ERDRP-0519 is a potent nonnucleoside inhibitor active against measles virus (MeV) and other Morbilliviruses. Conversely, polymerase inhibitors like ERDRP-0519 show greater promise due to the high conservation of the L-P complex across MeV strains. Here we report cryo-EM structures of the compound bound to MeV polymerase complexes at 2.73 Å and 2.48 Å resolution, revealing a unique binding pocket in the RdRp palm subdomain that overlaps the catalytic GDN motif. Structural analysis revealed that ERDRP-0519 binds to the palm subdomain of the RdRp, targeting the catalytic GDN motif and a nearby hydrophobic channel.

To test this, we assembled the MeV ternary polymerase complex14 with ERDRP-0519 and analyzed it by cryo-EM. The maps revealed two complexes: Lcore-P and Lfull-P-C, with clear ERDRP-0519 density on the L protein. Contrary to predictions, ERDRP-0519 was observed binding within the RdRp domain rather than at the predicted PRNTase site. First, it inhibits the catalytic center by interacting with residue D773 in the GDN motif. The piperidine group displaces D773, creating space for hydrophobic interaction that directly impairs active site function. A strong hydrogen bond (2.8 Å) forms between the compound’s carboxyl group in the linker and residue W671 of the L protein. ERDRP-0519 failed to inhibit the W671F mutant, confirming W671’s essential role in binding and antiviral activity. The central ring forms strong hydrophobic interactions with residue Y667, so any changes at this position are likely to cause steric clashes, disrupting binding. Additionally, the trifluoromethylated pyrazole group fits precisely into a hydrophobic pocket, engaging six surrounding residues and forming more interactions than any other part of the molecule.

> MDSLSVNQILYPEVHLDSPIVTNKIVAILEYARVPHAYSLEDPTLCQNIKHRLKNGFSNQMIINNVEVGNVIKSKLRSYPAHSHIPYPNCNQDLFNIEDKESTRKIRELLKKGNSLYSKVSDKVFQCLRDTNSRLGLGSELREDIKEKVINLGVYMHSSQWFEPFLFWFTVKTEMRSVIKSQTHTCHRRRHTPVFFTGSSVELLISRDLVAIISKESQHVYYLTFELVLMYCDVIEGRLMTETAMTIDARYTELLGRVRYMWKLIDGFFPALGNPTYQIVAMLEPLSLAYLQLRDITVELRGAFLNHCFTEIHDVLDQNGFSDEGTYHELIEALDYIFITDDIHLTGEIFSFFRSFGHPRLEAVTAAENVRKYMNQPKVIVYETLMKGHAIFCGIIINGYRDRHGGSWPPLTLPLHAADTIRNAQASGDGLTHEQCVDNWKSFAGVKFGCFMPLSLDSDLTMYLKDKALAALQREWDSVYPKEFLRYDPPKGTGSRRLVDVFLNDSSFDPYDVIMYVVSGAYLHDPEFNLSYSLKEKEIKETGRLFAKMTYKMRACQVIAENLISNGIGKYFKDNGMAKDEHDLTKALHTLAVSGVPKDLKESHRGGPVLKTYSRSPVHTSTRNVRAAKGFIGFPQVIRQDQDTDHPENMEAYETVSAFITTDLKKYCLNWRYETISLFAQRLNEIYGLPSFFQWLHKRLETSVLYVSDPHCPPDLDAHIPLYKVPNDQIFIKYPMGGIEGYCQKLWTISTIPYLYLAAYESGVRIASLVQGDNQTIAVTKRVPSTWPYNLKKREAARVTRDYFVILRQRLHDIGHHLKANETIVSSHFFVYSKGIYYDGLLVSQSLKSIARCVFWSETIVDETRAACSNIATTMAKSIERGYDRYLAYSLNVLKVIQQILISLGFTINSTMTRDVVIPLLTNNDLLIRMALLPAPIGGMNYLNMSRLFVRNIGDPVTSSIADLKRMILASLMPEETLHQVMTQQPGDSSFLDWASDPYSANLVCVQSITRLLKNITARFVLIHSPNPMLKGLFHDDSKEEDEGLAAFLMDRHIIVPRAAHEILDHSVTGARESIAGMLDTTKGLIRASMRKGGLTSRVITRLSNYDYEQFRAGMVLLTGRKRNVLIDKESCSVQLARALRSHMWARLARGRPIYGLEVPDVLESMRGHLIRRHETCVICECGSVNYGWFFVPSGCQLDDIDKETSSLRVPYIGSTTDERTDMKLAFVRAPSRSLRSAVRIATVYSWAYGDDDSSWNEAWLLARQRANVSLEELRVITPISTSTNLAHRLRDRSTQVKYSGTSLVRVARYTTISNDNLSFVISDKKVDTNFIYQQGMLLGLGVLETLFRLEKDTGSSNTVLHLHVETDCCVIPMIDHPRIPSSRKLELRAELCTNPLIYDNAPLIDRDATRLYTQSHRRHLVEFVTWSTPQLYHILAKSTALSMIDLVTKFEKDHMNEISALIGDDDINSFITEFLLIEPRLFTIYLGQCAAINWAFDVHYHRPSGKYQMGELLSSFLSRMSKGVFKVLVNALSHPKIYKKFWHCGIIEPIHGPSLDAQNLHTTVCNMVYTCYMTYLDLLLNEELEEFTFLLCESDEDVVPDRFDNIQAKHLCVLADLYCQPGTCPPIQGLRPVEKCAVLTDHIKAEAMLSPAGSSWNINPIIVDHYSCSLTYLRRGSIKQIRLRVDPGFIFDALAEVNVSQPKIGSNNISNMSIKAFRPPHDDVAKLLKDINTSKHNLPISGGNLANYEIHAFRRIGLNSSACYKAVEISTLIRRCLEPGEDGLFLGEGSGSMLITYKEILKLSKCFYNSGVSANSRSGQRELAPYPSEVGLVEHRMGVGNIVKVLFNGRPEVTWVGSVDCFNFIVSNIPTSSVGFIHSDIETLPDKDTIEKLEELAAILSMALLLGKIGSILVIKLMPFSGDFVQGFISYVGSHYREVNLVYPRYSNFISTESYLVMTDLKANRLMNPEKIKQQIIESSVRTSPGLIGHILSIKQLSCIQAIVGDAVSRGDINPTLKKLTPIEQVLINCGLAINGPKLCKELIHHDVASGQDGLLNSILILYRELARFKDNQRSQQGMFHAYPVLVSSRQRELISRITRKFWGHILLYSGNRKLINKFIQNLKSGYLILDLHQNIFVKNLSKSEKQIIMTGGLKREWVFKVTVKETKEWYKLVGYSALIKD;>MAEEQARHVKNGLECIRALKAEPIGSLAIEEAMAAWSEISDNPGQERATCREEKAGSSGLSKPCLSAIGSTEGGAPRIRGQGPGESDDDAETLGIPPRNLQASSTGLQCHYVYDHSGEAVKGIQDADSIMVQSGLDGDSTLSGGDNESENSDVDIGEPDTEGYAITDRGSAPISMGFRASDVETAEGGEIHELLRLQSRGNNFPKLGKTLNVPPPPDPGRASTSGTPIKKGTDARLASFGTEIASSLTGGATQCARKSPSEPSGPGAPAGNVPECVSNAALIQEWTPESGTTISPRSQNNEEGGDHYDDELFSDVQDIKTALAKIHEDNQKIISKLESLLLLKGEVESIKKQINRQNISISTLEGHLSSIMIAIPGLGKDPNDPTADVEINPDLKPIIGRDSGRALAEVLKKPVASRQLQGMTNGRTSSRGQLLKEFQLKPIGKKMSSAVGFVPDTGPASRSVIRSIIKSSRLEEDRKRYLMTLLDDIKGANDLAKFHQMLMKIIMKSG[4x]> E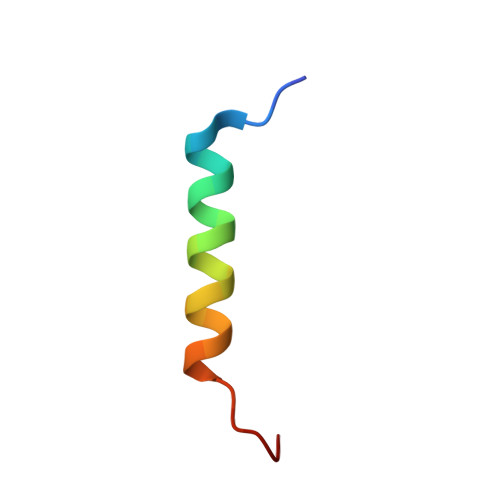YIKDCVFKDWEELGEEIRLKVFVLG> GSSSPPSPPLDLHVTDAGRKHIAIAWKPPEKNGGSPIIGYHVEMCPVGTEKWMRVNSRPIKDLKFKVEEGVVPD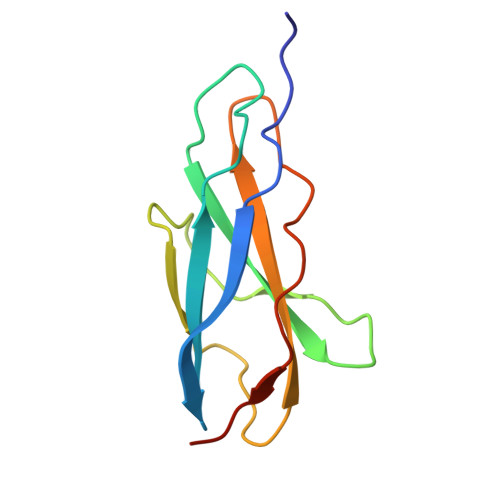KEYVLRVRAVNAIGVSEPSEISENVVAKDPDCK>[3x]QP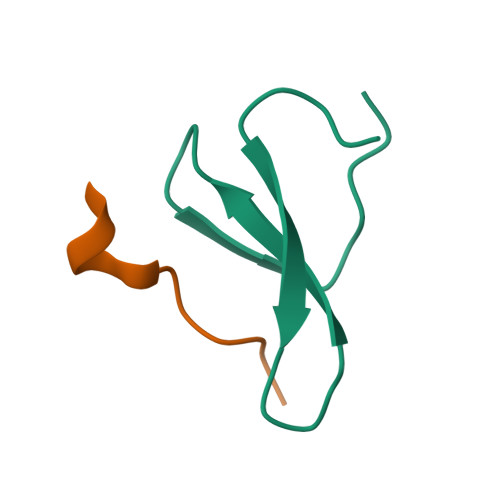HMPGLPSGWEERKDAKGRTYYVNHNNRTTTWTRPIM;>MEHRGPPPEYPFKGM[3x]> MGSSHHHHHHSNDPMSRQANRGTESKKMSSELFTLTYGALVTQLCKDYENDEDVNKQLDKMGFNIGVRLIEDFLARSNVGRCHDFRETADVIAKVAFKMYLGITPSITNWSPAGDEFSLILENNPLVDFVELPDNH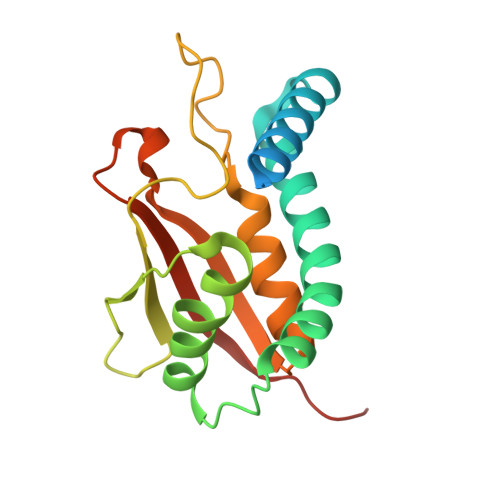SSLIYSNLLCGVLRGALEMVQMAVEAKFVQDTLKGDGVTEIRMRFIRRIEDNLPAGEE> VKEKLNGI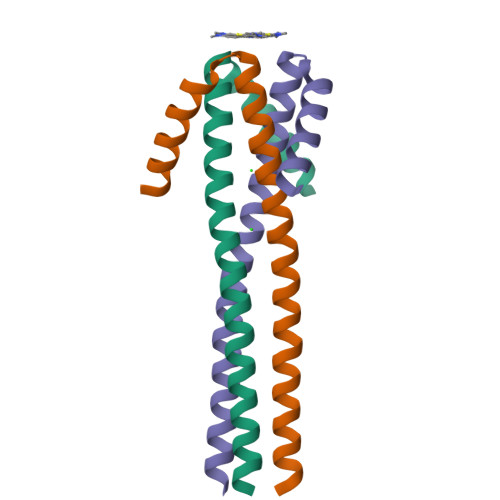IDQINKVNLLLEGEIEAVRRIAYMNQASSLQNQVEIGLIGEYLNISSWLETKTLTKTEEGLM> GMSDDLTDAQTAAIPEGFSQLNWSRGFGRQIGPLFEHREGPGQA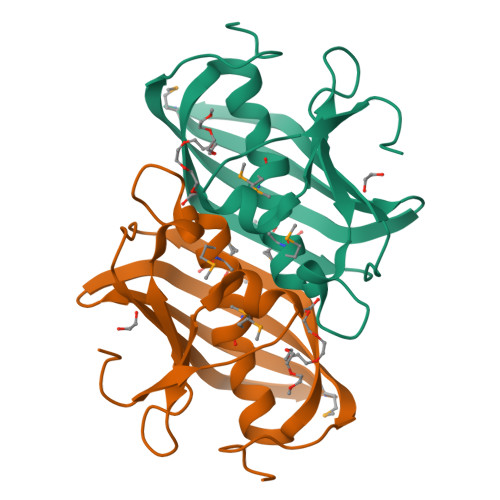RLAFRVEEHHTNGLGNCHGGMLMSFADMAWGRIISLQKSYSWVTVRLMCDFLSGAKLGDWVEGEGELISEEDMLFTVRGRIWAGERTLITGTGVFKALSARKPRPGELAYKEEA>MAHHHHHHSSGLEVLFQGPMIEIPSAATASPQYPQRRACPYRPAGGYERPVTRVRLYDGRPAWLVTGHETARQVLLDAATFSSDRQHPAFPALAARFEAARAVRNFIGMDPPEHTAQRRMLISGFTAKRVATLRPAITEIVDSLLDEVVRRGPGVDLVATFTLPVPSVVICRLLGVPYADHEFFEHQSRRIAAGTSTAAESADAFGQLKRYLLGLIETKGRGGEDMLDVLVDEQVATGTVTTPDLVDLALLLLVAGHETTASTLALGVALLLEQDGGAVAADPTRVGAVVEEILRHTAVADGVARFATRDTEVAGVRIAAGDAVVVALSAANRDPGPFPDPDRFDPRRGGRQHVTFGHGPHQCIGANLARAELEIALSRLFTRLPTLALAVPVEELGGKEAGGVQGVQRLPVTW[2x]

Using a combination of synthesis and in vitro assays we reveal that AbyV, a cytochrome P450 enzyme from the aby gene cluster, catalyses a key late‐stage epoxidation required for the installation of the characteristic ether‐bridged core of abyssomicin C. The X‐ray crystal structure of AbyV has been determined, which in combination with molecular dynamics simulations provides a structural framework for our functional data. Abyssomicin C is a spirotetronate antibiotic produced by the marine bacterium Micromonospora maris (originally Verrucosispora maris, reclassified in 2018). It is a potent inhibitor of bacterial folate metabolism, showing activity against a variety of clinically relevant bacterial pathogens including Mycobacterium tuberculosis and multi‐drug resistant strains of Staphylococcus aureus. In summary, here we report the first structural and functional characterisation of the enzyme AbyV and unambiguously establish its role in abyssomicin C biosynthesis. This cytochrome P450 is responsible for epoxidation of spirocycle 3, the penultimate step in the biosynthetic pathway and is key to installing the ether bridged core of abyssomicin C, a structural feature critical to its mechanism of action as a substrate mimetic of chorismate.

The crystal structure of AbyV reveals an asymmetric unit comprising two molecules of the polypeptide (Chains A and B), with Chain A accounting for residues 11–395 of the full‐length protein and Chain B residues 27–395. Electron density was not observed for residues 81–87 of Chain A and 73–94 of Chain B, consistent with the assignment of this region as the highly flexible BC loop. The overall fold of AbyV is typical of a cytochrome P450 with a large α‐helical domain (helices B–L) and a smaller β‐sheet region. Surprisingly, the region corresponding to helix “A” in other P450s forms a loop in AbyV, hence our assignment of the first helix of AbyV as “B”. Each molecule of AbyV contains a single heme group situated within a large solvent exposed active site pocket of ≈1600 Å3, as calculated using CASTp. The heme cofactor of AbyV is coordinated by the side chain of residue Cys344, with a single water molecule observed on the opposing face of the cofactor, 2.1 Å above the heme iron. Each of the two molecules of AbyV that comprise the AU contain a single molecule of PEG bound within the enzyme active site. Our crystal structure provides no evidence for the presence of atypical catalytic features in AbyV such as those reported in other P450 enzymes. To explore the likely enzyme‐substrate interactions of both atropisomers of spirocycle 3, we used molecular docking to obtain initial positions of 3 near the heme group in chain A of the AbyV crystal structure.>MEPQETENTIEADAGIAGRAGGGGGPGGGGSGGGSGVGVSTGGWEGGTLFGDNRVITVNTRQWYAPIYNGHRYTKLEGTGNTFWKGIKTPWGYFNFNAYDSHFSPQDWQRLTNEYRRWRPKKMMVKIYNLQIKQVVTLQGDTLYNNDLTAGVHIFCDGSHQYPYSQHPWDAGTMPELPYKVWLLENYGYFQFQGDLIDTSVDGGSPDVENVEKEIAKSAPFYILENANHEVLRTGEETNFHFNFDCGWVNNDRAYCPLQADFNPLVKTRRYFATRNNYNNSGKFVYTRYSPYNKPSQWMPGPSLGYIGNTQSAATREQALGPVTVVTAPPGTSAYTAFTEQQSKTNQQSASNATWSGYDVSPVNCARSGFDKIGLAYDSAPESELEEKISIRDIDNDMSRWGQVFVQDGTNKEISNDNTGQGGNTRQNMAELKNVWMFPNQAWDSTPISRDFPIWVKSPNTDKHTLFDSSDGTLPMSHPPGTIFVKVAKIPIPTQTNTDS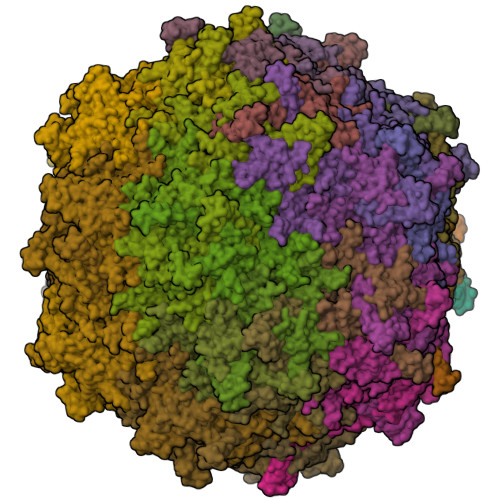YLTLYVTGQVTCTIEWEVERFMTKNWRPESKNDVSSFRDAFLYTVGADGTYNTPERFLEGMPTRRGINKTL[60x]2,3,5-trimethyl-6-[3-oxo-3-(piperidin-1-yl)propyl]-7H-furo[3,2-g][1]benzopyran-7-one 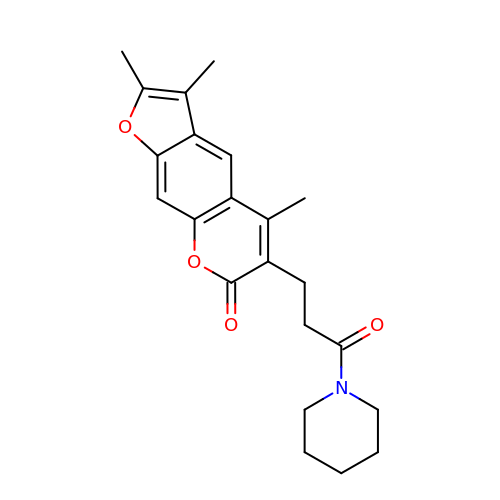| C22 H25 N O4 | SHGFQSFSJDFZLK-UHFFFAOYSA-N>[4x]DPGC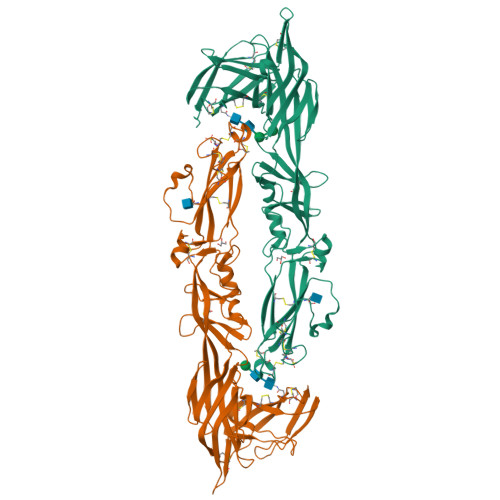SELIQASSRITTCSTEGVNTKCRLSGTALIRAGSVGAEACLMLKGVKEDQTKFLKIKTVSSELSCREGQSYWTGSFSPKCLSSRRCHLVGECHVNRCLSWRDNETSAEFSFVGESTTMRENKCFEQCGGWGCGCFNVNPSCLFVHTYLQSVRKEALRVFNCIDWVHKLTLEITDFDGSVSTIDLGASSSRFTNWGSVSLSLDAEGISGSNSFSFIESPGKGYAIVDEPFSEIPRQGFLGEIRCNSESSVLSAHESCLRAPNLISYKPMIDQLECTTNLIDPFVVFERGSLPQTRNDKTFAASKGNRGVQAFSKGSVQADLTLMFDNFEVDFVGAAVSCDAAFLNLTGCYSCNAGARVCLSITSTGTGSLSAHNKDGSLHIVLPSENGTKDQCQILHFTVPEVEEEFMYSCDGDERPLLVKGTLIAIDP> MLQSFADTVWLIPFYSLAGMVLSLIWSPGITRKTGPRPAGYLNILLTFFSFVHALLATVAIANQPPQYLHWTWLDVAGLHLDIPVEISILTTTALMLITALNLMAQVFAVGYMEMDWGWARFFALLALFEGGMGALVLLDSLFFNYVVLEILTLATYLLIGLWFNQPLVVTGARDAFLTKRVGDLVLLMGVLAIYPLAGSWNYDDLAAWAATAQVNSTLITLICLALIAGPMGKCAQFPLHLWLDEAMEGPIPASILRNAVVVATGAWVLVKLTP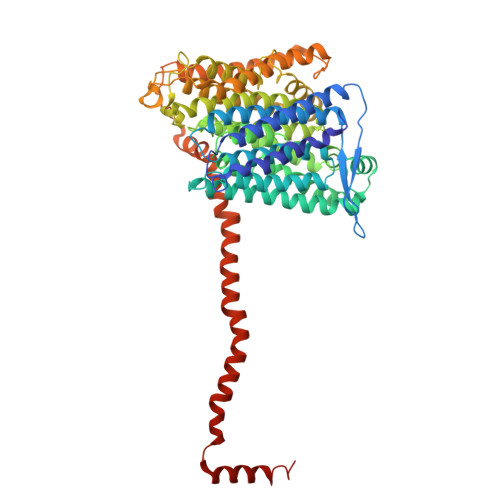VLSLSPVALTALLVIGSVTALGGTLIAIAQVDIKRALSYLVSAYMGWVFIAVGLKEPGLAFVFILTYSLAMAVLMMSIGSIIWNSVTQDLRLLGGLWSRRPISGISFLVGSAGLLAVPPLASFFPQAELLDTAFAQLPWVGGVLLLMNTFAAFSLGRTFCLVWGGEVKPMTARSPEVFWPMILPMTVDLGLVLHLPILMARFDWVIWTQPSLATAAALTITALLGWGVAAWVYLGKAIPKPVQFPLPSVQNLLAYDFYTPKLYRATVVGVVDMISRITAWFDRTFVDGTGNAFGVVTLLGGDRLKYSTTGQSQAYILTILMGIAILVIAICWPLLA>GTMGKSKGTRFERDLLVELWKAGFAAIRVAGSGVSPFPCPDIVAGNGRTYLAIEVKMRKELPL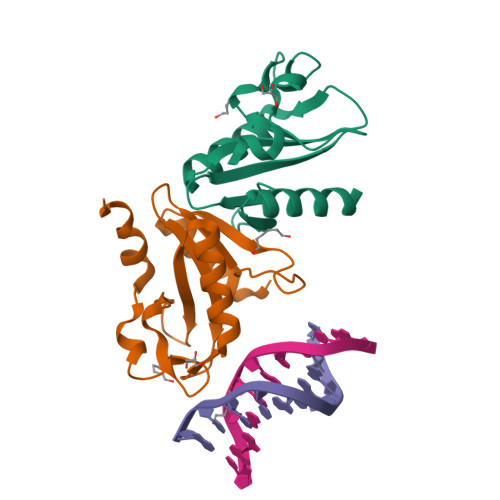YLSADEVEQLVTFARGFGAEAYVALKLPRKKWRFFPVQMLERTEKNFKIDESVYPLGLEIAEVAGKFFQERFGEKV[2x]>MSRGALIVFEGLDKSGKTTQCMNIMESIPANTIKYLNFPQRSTVTGKMIDDYLTRKKTYNDHIVNLLFCANRW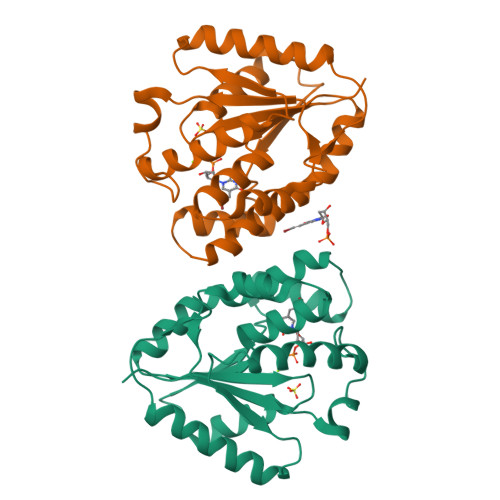EFASFIQEQLEQGITLIVDRYAFSGVAYAAAKGASMTLSKSYESGLPKPDLVIFLESGSKEINRNVGEEIYEDVTFQQKVLQEYKKMIEEGDIHWQIISSEFEEDVKKELIKNIVIEAIHTVTGPVGQLWM[2x]>[2x]QTSPPGWRELVPPDTLHSLPKSQVKRQEVISELLVTEAAHVRMLRVLHDLFFQPMAECLFFPLEELQNIFPSLD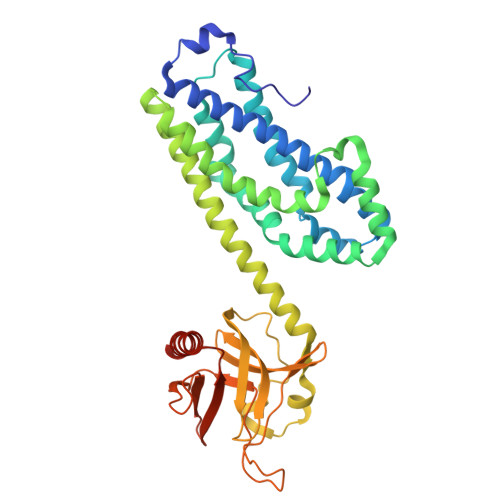ELIEVHSLFLDRLMKRRQESGYLIEEIGDVLLARFDGAEGSWFQKISSRFCSRQSFALEQLKAKQRKDPRFCAFVQEAESRPRCRRLQLKDMIPTEMQRLTKYPLLLQSIGQNTEEPTEREKVELAAECCREILHHVNQAVRDMEDLLRLKDYQRRLDLSHLRQSSDPMLSEFKNLDITKKKLVHEGPLTWRVTKDKAVEVHVLLLDDLLLLLQRQDERLLLKSHSRTLTPTPDGKTMLRPVLRLTSAMTREVATDHKAFYVLFTWDQEAQIYELVAQTVSERKNWCALITETAGSLKVPA>[4x]SHMTPKELLEWQTNWKKIMKRDSRIYFDITDDVEMNTYNKSKMDKRRDLLKRGFLTLGAQITQFFDTTVTIVITRRSVENIYLLKDTDILSRAKKNYMKVWSYEKAARFLKNLDVDLDHVDSGASGGSKFSQEQIGENIVCRVICTTGQIPIRDLSADISQVLKEKRSIKKVWTFGRNPACDYHLGNISRLSNKHFQILLGEDGNLLLNDISTNGTWLNGQKVEKNSNQLLSQGDEITVGVGVESDILSLVIFINDKFKQCLEQNKVDR

Rad53, and its mammalian ortholog the checkpoint kinase 2 (Chk2), are key effector kinases of the DNA replication checkpoint. Rad53 contains two forkhead-associated (FHA) domains, as well as two SQ/TQ cluster domains (SCD), flanking its kinase domain. The phosphoepitope-binding site recognizes an epitope present in DDK24, whereas one of the lateral surfaces of FHA1 interacts with the modified BRCT domain of Dbf416, herein referred to as HBRCT domain due to the presence of an additional α-helix at the N-terminus of the domain. We generated chimeras expressing the HBRCT (Dbf4) and FHA1 (Rad53) domains in tandem and solved the crystal structures of these chimeras in the absence and presence of a phosphorylated epitope derived from Cdc7.

Therefore, we anticipated that we could stabilize the interaction by producing the two domains as a single polypeptide chain. We fused the FHA1 domain of Rad53 at the C-terminus of the HBRCT domain of Dbf4 directly, or using a five-residue glycine/serine-rich linkers (Dbf4(0)Rad53 and Dbf4(5)Rad53; Fig. 1A). The chimera containing a five-residue linker readily yielded diffraction-quality crystals. The asymmetric unit contained four copies of the Dbf4(5)Rad53 chimera arranged to form four Dbf4:Rad53 complexes. The C-terminal end of Dbf4 (residues 216–220) and the N-terminal end of Rad53 (residues 22–29), as well as the five amino acid linker, were disordered in the structure. The distance between the last ordered residue of the HBRCT domain of Dbf4 and the first ordered residue in the closest FHA1 neighbors, the crystal packing contacts and the behavior in solution of the chimeras, confirms that the Dbf4:Rad53 complex forms inter-molecularly. Importantly, the four complexes in the asymmetric unit had identical interfaces, indicating that the linkers did not constrain complex formation. In good agreement with our previous results showing that the pThr-binding pocket of the FHA1 domain does not mediate the interaction with Dbf416, the complex forms through the lateral surface of the FHA1 domain defined by the β2-β1-β11-β10-β7-β8 strands and the concave surface of the HBRCT domain. On one side of the interface, the side chains of residues Arg35 (β1), Ile37 (β1), Val144 (β11) and Phe146 (β11) of Rad53 are cradled by the α0 helix of the HBRCT domain, specifically by residues Glu111, Trp112, Asn115 and Trp116, defining interface I. On the other side, the loop containing residues Tyr198 and Lys200 of Dbf4 wraps around the β7/β8 loop of the FHA1 domain enabling the interaction between the amine group of Lys200 and Asn112 (β7) in Rad53 defining interface II. Globally the two interfaces bury a mere 10% of the total accessible surface area of the FHA1 (755 out of 6,664 Å2) and the HBRCT (801 out of 7,799 Å2) domains, a value that is below the cutoff for specific interactions as judged using the PISA server33.6-((((3S, 5R)-5-(((6-amino-4-methylpyridin-2-yl)methoxy)methyl)pyrrolidin-3-yl)oxy)methyl)-4-methylpyridin-2-amine | C19 H27 N5 O2 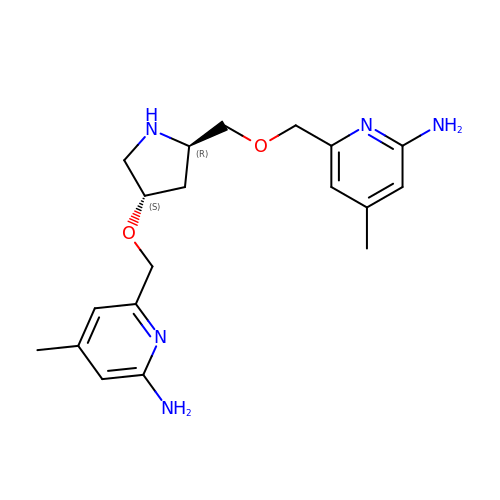| NUKSCYDKRQJOFO-PBHICJAKSA-N>MKTPWKVLLGLLGIAALVTVITVPVVLLNKGTDDAAADSRRTYTLTDYLKSTFRVKFYTLQWISDHEYLYKQENNILLFNAEYGNSSIFLENSTFDELGYSTNDYSVSPDRQFILFEYNYVKQWRHSYTASYDIYDLNKRQLITEERIPNNTQWITWSPVGHKLAYVWNNDIYVKNEPNLSSQRITWTGKENVIYNGVTDWVYEEEVFSAYSALWWSPNGTFLAYAQFNDTEVPLIEYSFYSDESLQYPKTVRIPYPKAGAENPTVKFFVVDTRTLSPNASVTSYQIVPPASVLIGDHYLCGVTWVTEERISLQWIRRAQNYSIIDICDYDESTGRWISSVARQHIEISTTGWVGRFRPAEPHFTSDGNSFYKIISNEEGYKHICHFQTDKSNCTFITKGAWEVIGIEALTSDYLYYISNEHKGMPGGRNLYRIQLNDYTKVTCLSCELNPERCQYYSASFSNKAKYYQLRCFGPGLPLYTLHSSSSDKELRVLEDNSALDKMLQDVQMPSKKLDVINLHGTKFWYQMILPPHFDKSKKYPLLIEVYAGPCSQKVDTVFRLSWATYLASTENIIVASFDGRGSGYQGDKIMHAINRRLGTFEVEDQIEATRQFSKMGFVDDKRIAIWGWSYGGYV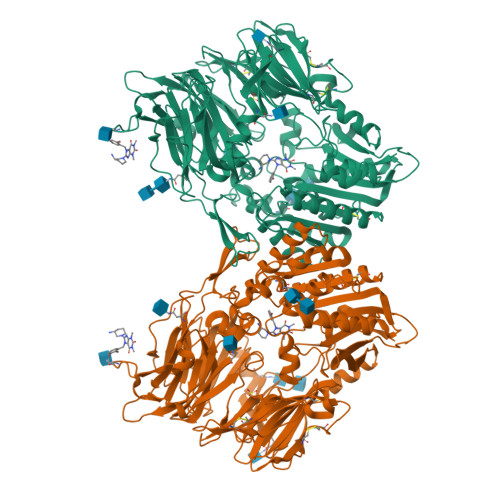TSMVLGAGSGVFKCGIAVAPVSKWEYYDSVYTERYMGLPTPEDNLDYYRNSTVMSRAENFKQVEYLLIHGTADDNVHFQQSAQLSKALVDAGVDFQTMWYTDEDHGIASNMAHQHIYTHMSHFLKQCFSLP[4x]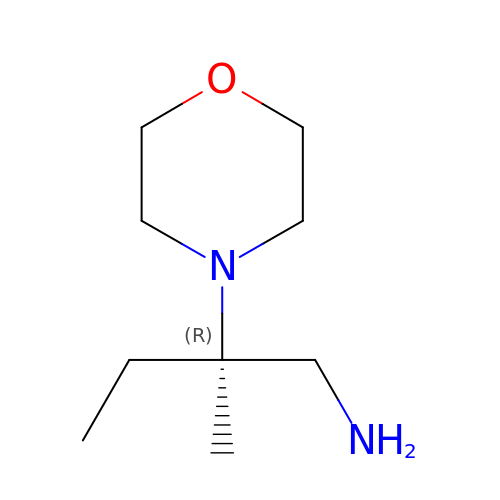(2R)-2-methyl-2-(morpholin-4-yl)butan-1-amine | C9 H20 N2 O | RNGALZNABGSEIF-SECBINFHSA-N> MLPSFLLSSLLCLSTVSALPNPIIAERAACDCTGTRDGGSSSKDYICRDARLGPTKLPKKLPLSATVESYNRFGGLTPIQFLQTWTDEKGNYKYPPQNGFQLDANGN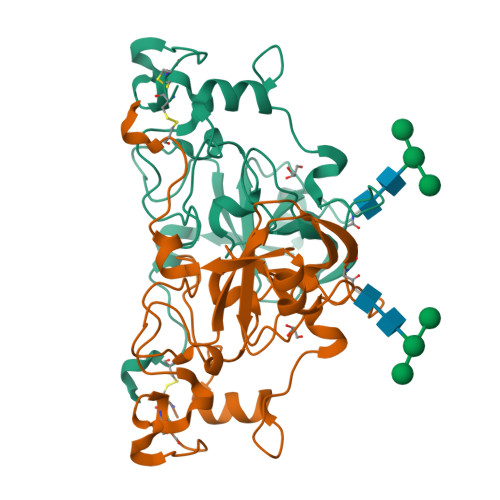AINGSMVLQVGTLVDRFGSEYGSYVSAASAPYSQRALPPSNLATNPDTPDFPYNYHVYRVIKPLTVVGGPIAPWFGQPGLGAQFFTGETGNVKFLIEQNYLQKEDPSALVYKSDGCADVLFQ>[8x]AVPAPNQQPEVFCNQIFINNEWHDAVSRKTFPTVNPSTGEVICQVAEGDKEDVDKAVKAARAAFQLGSPWRRMD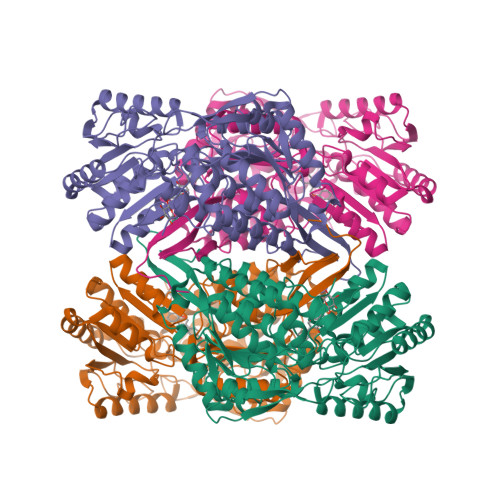ASHRGRLLNRLADLIERDRTYLAALETLDNGKPYVISYLVDLDMVLKCLRYYAGWADKYHGKTIPIDGDFFSYTRHEPVGVCGQIIPWNFPLLMQAWKLGPALATGNVVVMKVAEQTPLTALYVANLIKEAGFPPGVVNIVPGFGPTAGAAIASHEDVDKVAFTGSTEIGRVIQVAAGSSNLKRVTLELGGKSPNIIMSDADMDWAVEQAHFALFFNQGQCCCAGSRTFVQEDIYDEFVERSVARAKSRVVGNPFDSKTEQGPQVDETQFKKILGYINTGKQEGAKLLCGGGIAADRGYFIQPTVFGDVQDGMTIAKEEIFGPVMQILKFKTIEEVVGRANNSTYGLAAAVFTKDLDKANYLSQALQAGTVWVNCYDVFGAQSPFGGYKMSGSGRELGEYGLQAYTEVKTVTVKVPQKNS>GSGEGSEDD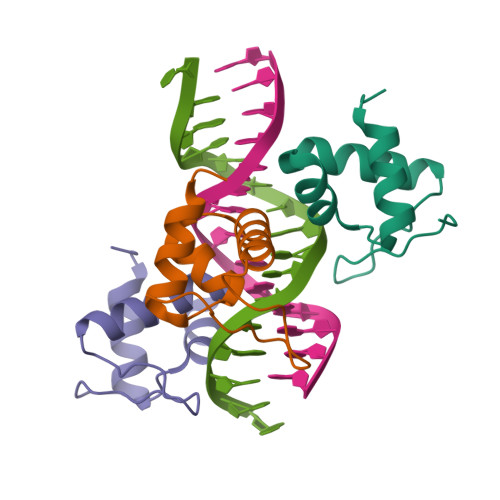PLYDEAVRFVTESRRASISAVQRKLKIGYNRAARMIEAMEMAGVVTPMNTNGSREVIAPAPVRD[6x]> ERAGPVTWVMMIACVVVFIAMQILGDQEVMLWLAWPFDPTLKFEFWRYFTHALMHFSLMHILFNLLWWWYLGGAVEKRLGSGKLIVITLISALLSGYVQQKFSGPWFGG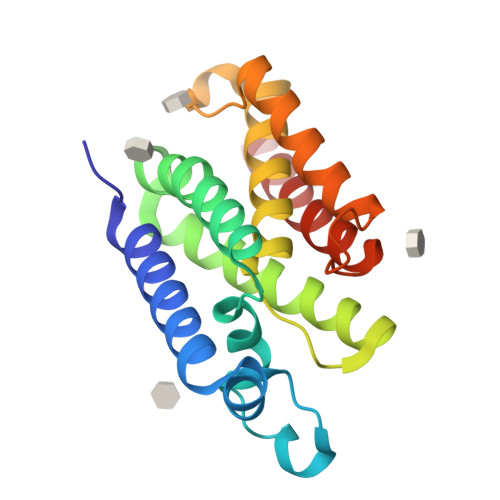LTGVVYALMGYVWLRGERDPQSGIYLQRGLIIFALIWIVAGWFDLFGMSMANGAHIAGLAVGLAMAFVDSLN>GSHMMPGEIRPTIGQQMETGDQRFGDLVFRQLAPNVWQHTSYLDMPGFGAVASNGLIVRDGGRVLVVDTAWTDDQTAQILNWIKQEINLPVALAVVTHAHQDKMGGMDALHA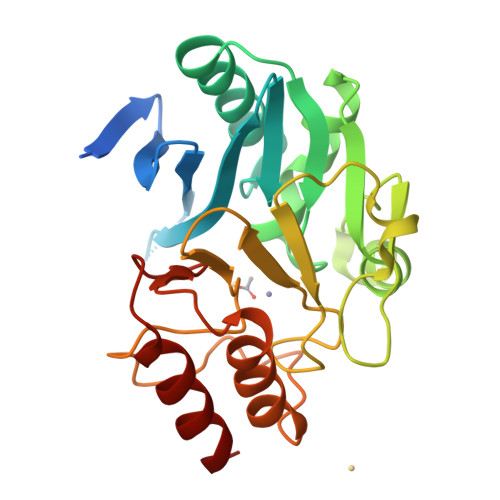AGIATYANALSNQLAPQEGMVAAQHSLTFAANGWVEPATAPNFGPLKVFYPGPGHTSDNITVGIDGTDIAFGGCLIKDSKAKSLGNLGDADTEHYAASARAFGAAFPKASMIVMSHSAPDSRAAITHTARMADKLR[2x];> CPFPEPKL> GSHMRQHVFLVSEYLKDASKKMKNGLMFVKLVNPCSGEGAIYLFNMCLQQLFEVKVFKEKHHSWFINQSVQSGGLLHFATPVDPLFLLLHYLIKADKEGKFQPLDQVVVDNVFPNCILLLKLPGLEKLLHHVTEEKG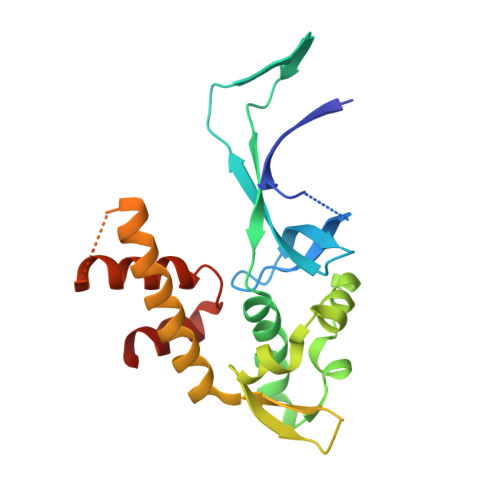NPEIDNKKYYKYSKEKTLKWLEKKVNQTVAALKTNNVNVSSRVQSTAFFSGDQASTDKEEDYIRYAHGLISDYIPKELSDDLSKYLK Outer mitochondrial membrane (OMM) fusion is catalyzed by the dynamin-like GTPase called mitofusin (MFN). We generated a modified human MFN2 construct with deletions of residues 1–21 and 401–705 (MFN2IM). MFN2IM contains a G domain and a helical domain 1 (HD1). In this study, we address these issues by presenting crystal structures of truncated human MFN2 in different stages of the GTP turnover cycle. These structures explain how MFN2 uses a primate-only single amino acid variance and a tighter G interface, as compared with human MFN1, to allow for enduring GTPase (G) domain association even after GTP hydrolysis, a feature that is unique in the dynamin superfamily and ensures efficient membrane tethering.

For the MFN2IM crystals that yielded the GDP-bound structure, the GDP was not added during purification or crystallization, but co-purified from the host E. coli cells. Somewhat unexpectedly, this GDP-bound MFN2IM forms a G domain-mediated dimer across the asymmetric units of the crystal lattice. RALS analysis revealed that the majority of freshly purified MFN2IM molecules were indeed in the dimeric form. These observations indicate that MFN2IM dimerizes during GTP hydrolysis, and the dimer remained associated after the reaction. In the crystal structure, two citrate ions were present between the associated G domains, and making contacts with both of them in a symmetrical manner. In solution, however, citrate did not affect GTP hydrolysis, or induce dimerization of GDP-bound MFN2IM, suggesting that the MFN2IM-GDP dimer in the crystal structure is not dependent on citrate. By comparing the catalytic sites between our MFN2IM-GDP structure and MFN1IM in the transition state (MFN1IM-GDP∙BeF3−), we found that their switch I regions are very similar in overall conformations, as are the positions of the catalytic threonine. On the G interface of MFN2IM, the trans interactions include (i) the central dual salt bridges between Glu230 and Arg259; (ii) a hydrophobic cluster involving Ile126 on switch I and Trp260/Val273, and (iii) other hydrogen bonds and salt bridges. Thus, our MFN2IM-GDP dimer may represent a posttransition state right after GTP hydrolysis. More importantly, Glu266 forms an MFN2-specific trans salt bridge to Lys307, whose side chain is in parallel with the guanine group of the nucleotide. This association, together with the central salt bridge and η1G, tightly enwraps the nucleotide.

> GPHMGGSAEVNASPLKHFVTAKKKINGIFEQLGAYIQESATFLEDTYRNAELDPVTTEEQVLDVKGYLSKVRGISEVLARRHMKVAFFGRTSNGKSTVINAMLWDKVLPSGIGHTTNCFLRVEGTDGHEAFLLTEGSEEKRSAKTVNQLAHALHQDKQLHAGSLVSVMWPNSKCPLLKDDLVLMDSPGIDVTTELDSWIDKFCLDADVFVLVANSESTLMQTEKHFFHKVSERLSRPNIFILNNRWDASASEPEYMEEVRRQHMERCTSFLVDELGVVDRSQAGDRIFFVSAKEVLNARIQKAQGMPEGGGALAEGFQVRMFEFQNFERRFEECISQSAVKTKFEQHTVRAKQIAEAVRLIMDSLHMAAREQQVYCEEMREERQDRTRENLEQEIAAMNKKIEVLDSLQSKAKLLRNKAGWLDSELNMFTHQYLQPSR>CTAITLNGNSNYFGRNLDLDFSYGEEVIITPAEYEFKFRKEKAIKNHKSLIGVGIVANDYPLYFDAINEDGLGMAGLNFPGNAYYSDALENDKDNITPFEFIPWILGQCSDVNEARNLVEKINLINLSFSEQLPLAG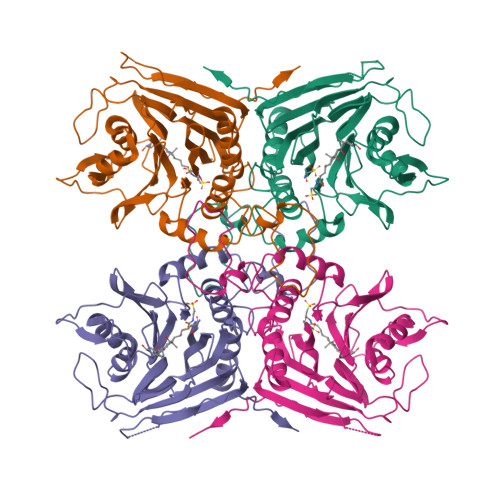LHWLIADREKSIVVEVTKSGVHIYDNPIGILTNNPEFNYQMYNLNKYRNLSISTPQNTFSDSVDLKVDGTGFGGIGLPGDVSPESRFVRATFSKLNSSKGMTVEEDITQFFHILGTVEQIKGVNKTESGKEEYTVYSNCYDLDNKTLYYTTYENRQIVAVTLNKDKDGNRLVTYPFERKQIINKLNLE[8x]>ACVFACEDAAIIG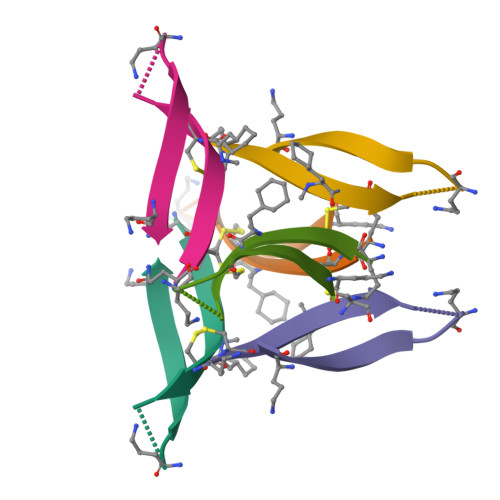LAV[4x]2-(BENZOYLAMINO)ETHANESULFONIC 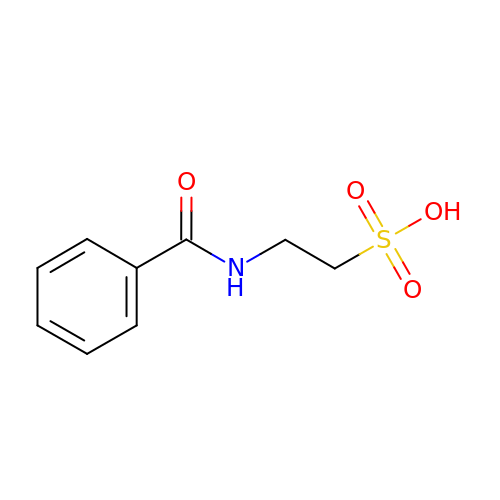ACID | C9 H11 N O4 S | ABUKAMCDAHVPSR-UHFFFAOYSA-N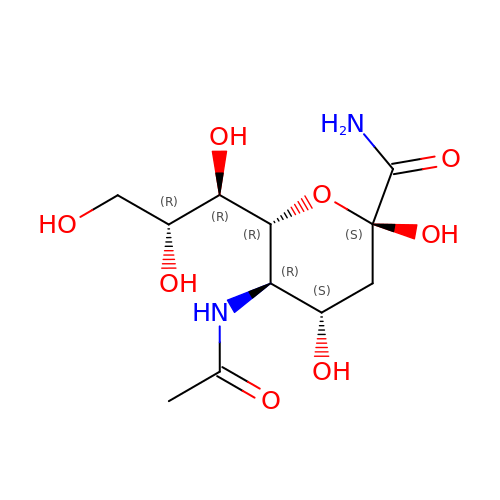(2S,4S,5R,6R)-5-acetamido-2,4-dihydroxy-6-[(1R,2R)-1,2,3-trihydroxypropyl]oxane-2-carboxamide | C11 H20 N2 O8 | PKSULYZGXFBQIQ-PFQGKNLYSA-N> YCQKWMWTCDSE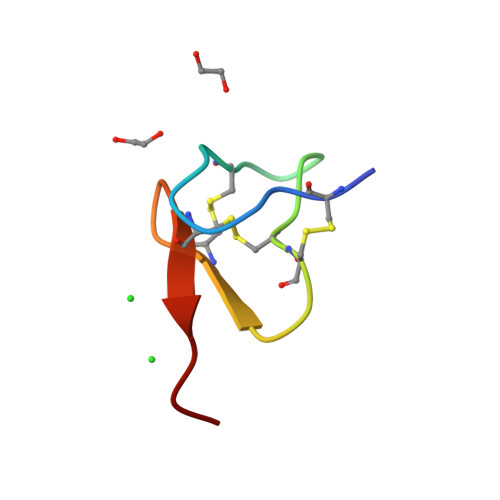RKCCEGMVCRLWCKKKLW> MAKTVAYFYDPDVGNFHYGAGHPMKPHRLALTHSLVLHYGLYKKMIVFKPYQASQHDMCRFHSEDYIDFLQRVSPTNMQGFTKSLNAFNVGDDCPVFPGLFEFCSRYTGASLQGATQLNNKICDIAINWAGGLHHAKKFEASGFCYVNDIVIGILELLKYHPRVLYIDIDIHHGDGVQEAFYLTDRVMTVSFHKYGNYFFPGTGDMYEVGAESGRYYCLNVPLRDGIDDQSYKHLFQPVINQVVDFYQPTCIVLQCGADSLGCDRLGCFNLSIRGHGECVEYVKSFNIPLLVLGGGGYTVRNVARCWTYETSLLVEEAISEELPYSEYFEYFAPDFTLHPDVSTRIENQNSRQYLDQIRQTIFEN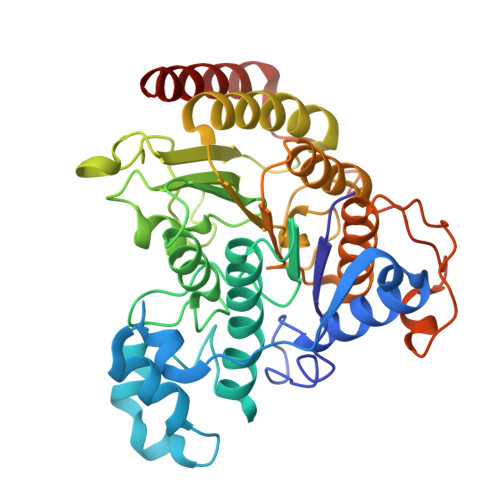LKMLNHAPSVQ>[10x]QANLMRLKSDLFNRSPMYPGPTKDDPLTVTLGFTLQDIVKVDSSTNEV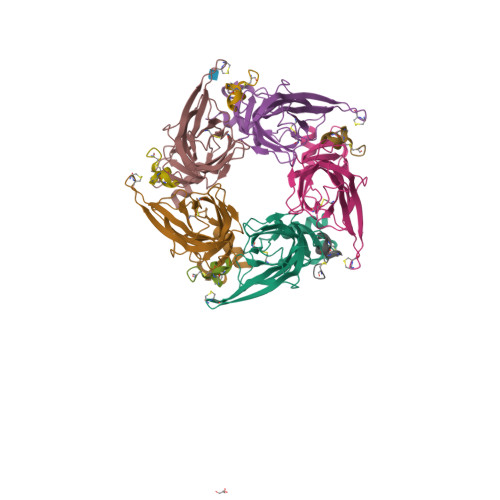DLVYYEQQRWKLNSLMWDPNEYGNITDFRTSAADIWTPDITAYSSTRPVQVLSPQIAVVTHDGSVMFIPAQRLSFMCDPTGVDSEEGVTCAVKFGSWVYSGFEIDLKTDTDQVDLSSYYASSKYEILSATQTRQVQHYSCCPEPYIDVNLVVKFRERRAGNGFFRNLFD;>GCCSRPPCILNNPDLCX[10x]>[2x]AHMSTGEAIPRVAVVVFILNGNSILLGRRRSSIGNSTFALPGGHL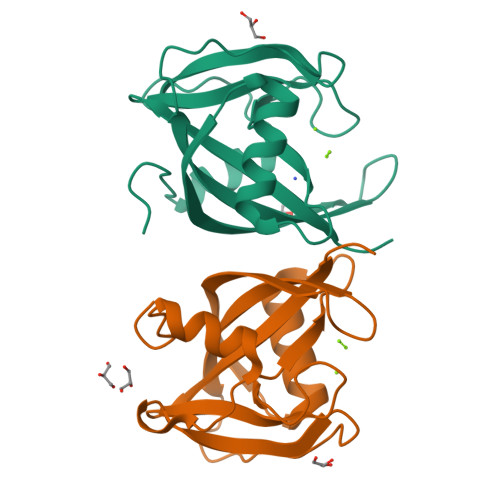EFGESFEECAAREVMEETGLKIEKMKLLTVTNNVFKEAPTPSHYVSVSIRAVLVDPSQEPKNMEPEKCEGWDWYDWENLPKPLFWPLEKLFGSGFNPFTHGGGD> MGHHHHHHMKEPTQMVYSVGLTGNIASGKSTVAEFFSELGINVIYADKIAKELTSKNTPCYQDIISHFGSSVVLNNGELDRKRIR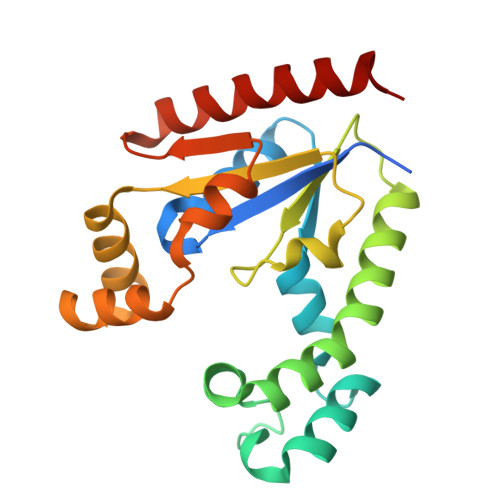DIIFSNSNERLWLESLLHPVIRKKIEEQLIVCTSPYCLIEIPLLFNKHHYPYLQKVLLVIAPLESQLDRIVKRDHCTKKQALAILATQPNLEQRLEAADDVLINESGLSELKAKVNKLHQKYLREAKIKQ>ASGLVASNLNLKPGECLR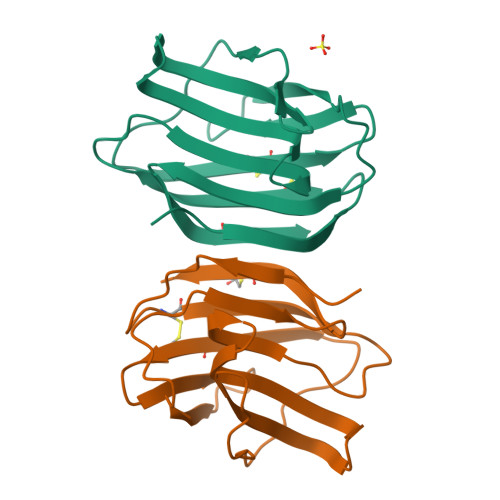VRGEVAPDAKSFVLNLGKDSNNLCLHFNPRFNAHGDANTIVCNSKDDGAWGTEQREAVFPFQPGSVAEVCITFDQANLTVKLPDGYEFKFPNRLNLEAINYMAADGDFKIKCVAFD[2x]> MAPTWFYNTTNSEKLRELQHVLGGSAKLGYLTAKVTEILDVDLETVIRAKAIAAYRAVRVPVIVEHGALCIDALNGLPGALVKPFWESLDTRLCEVIPAGQRTARARGALCYCDGRERHVLI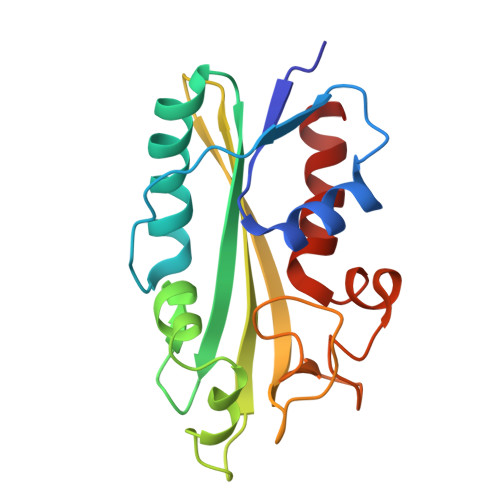EETEGEIAPSARGTGGFHWDPIFIPKGQTRTFAEMSLDEKLSFSPLGRLHTRLRTELGL> TVETKELNQPLDVVVLLDNSNSMNNERANNSQRALKAGEAVEKLIDKITSNKDNRVALVTYASTIFDGTEATVSKGVADQNGKALNDSVSWDYHKTTFTATTHNYSYLNLTNDANEVNILKSRIPKEAEHINGDRTLYQFGATFTQKALMKANEILETQSSNARKKLIFHVTDGVPTMSYAINFNPYISTSYQNQFNSFLNKIPDRSGILQEDFIINGDDYQIVKGDGESFKLFSDRKVPVTGGTTQAAYRVPQNQLSVMSNEGYAINSGYIYLYWRDYNWVYPFDPKTKKVSATKQIKTHGEPT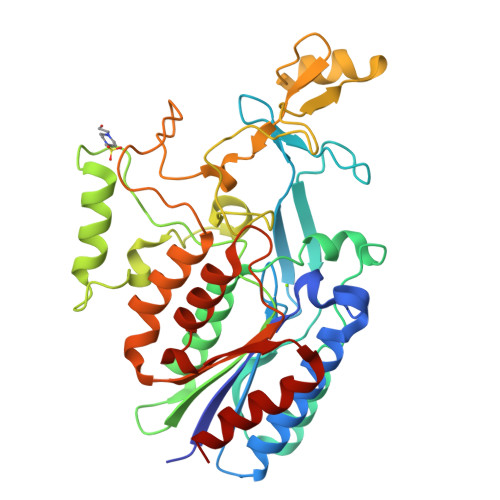TLYFNGNIRPKGYDIFTVGIGVNGDPGATPLEAEKFMQSISSKTENYTNVDDTNKIYDELNKYFKTIV>[10x]AGHMSLYRLIYSSQGIPNLQPQDLK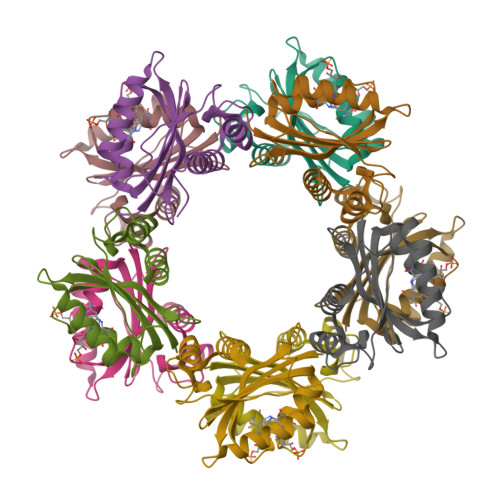DILESSQRNNPANGITGLLCYSKPAFLQVLEGECEQVNETYHRIVQDERHHSPQIIECMPIRRRNFEVWSMQAITVNDLSTEQVKTLVLKYSGFTTLRPSAMDPEQCLNFLLDIAKIYELSDNFFLDL> GSHMGSRPLPLADLARLLDAVQGRIQVASAAESHAARLQVRLPQLGAVEVQVLHGHGQLQIEISASPGSLALLQQARGELLERLQRLHPEQPVQLTFNQ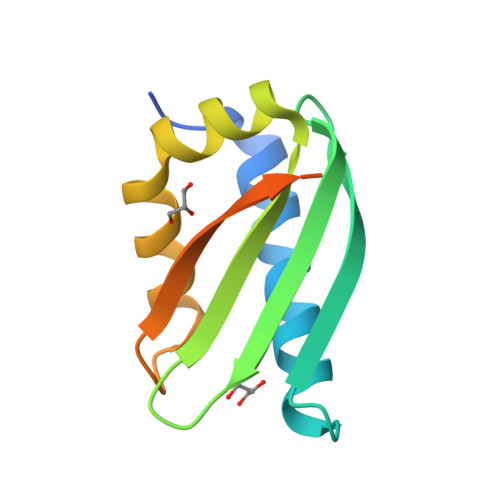QQDSGQRSRQRRYLHEEWQAE> MQPFYEEYRKAWNQINDHIADLQHRSY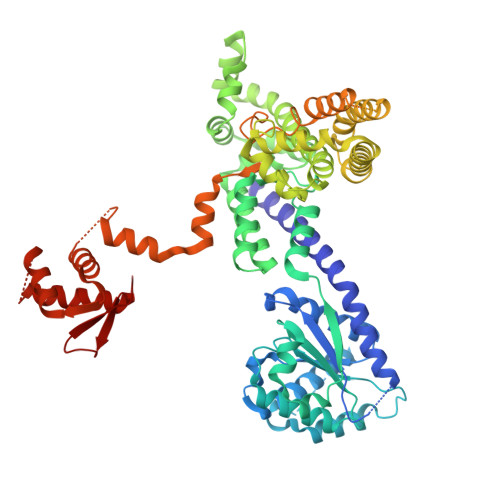ARTLEQLVDFVVGQAERDTPDEVLPTAALLTGINQPDHLSQFTALTQRLHAQRAAMVCVLQSRDCATLKAAVETLVFGLVEDNAEVEQMEDEDEDEDGAERDRKRLRRSQCTMKQLKSWYTNNFDSEQKRRQLVVILPDFECFNASVLQDLILILSAHCGSLPFVLVLGVATAMTAVHGTLPYHVSSKIRLRVFQTQAAPTGLNEVLDKVLLSPKYAFHLSGKTFKFLTHIFLYYDFSIHGFIQGFKYCLMEHFFGGNAFALCTDYSKALGRIKQLTHEDMETIRRLPSFRPYVEQINDCKRIIAVLTDDDYLKKKLPQLLRDCLLHFLLFRCSLEFLTELVGDLPRCPLGKLRRELYVNCLNRAIISTPEYKECLQMLSFLSKDEFVAKVNRALERTEQFLVEEIAPLELGEACTAVLRPKLEAIRLAVDEVVKATMATITTTSPNETRQATDHLTPVASRQELKDQLLQRSKEDKMRHQLNTPTTQFGRALQKTLQLIETQIVQDHLRALQDAPPIHELFVFSDIATVRRNIIGAPRAALHTALNNPHFYMQCKCCELQDQSLLVGTLPDLSVVYKLHLECGRMINLFDWLQAFRSVVSDSDHEEVAQEQIDPQIQARFTRAVAELQFLGYIKMSKRKTDHATRLTW> MTDSVQTETTEGKIIINLFAPNLPGSTKEDDLIQKSLRDQLVESIRNSIAYPDTDKFAGLTRFIDESGRNVFFVDGTRGAGKTTFINSVVKSLNSDQDDVKVNIKCLPTIDPTKLPRHEPILVTVTARLNKMVSDKLKGYWASNDYRKQKEQWQNHLAQLQRGLHLLTDKEYKPEYFSDALKLDAQLDYSIGGQDLSEIFEELVKRACEILDCKAILITFDDIDTQFDAGWDVLESIRKFFNSRKLVVVATGDLRLYSQLIRGKQYENYSKTLLEQEKESVRLAERGYMVEHLEQQYLLKLFPVQKRIQLKTMLQLVGEKGKAGKEEIKVKTEPGMQDIDAIDVRQAIGDAVREGLNLREGSDADMYVNELLK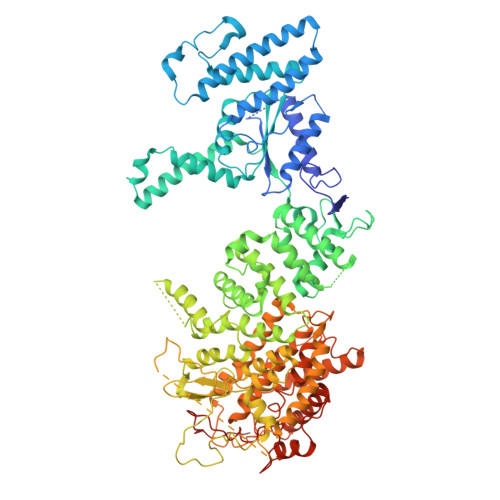QPVRLLMQVLQDFYTKKYHATSVKLDGKQSRNERPNELSVPNLLRNALYGSMLSSIYRAGLNYEQHRFGMDSLCKDIFTYVKQDRDFNTGFYLRPQSESEALRNCSIYLASQVSENCQGSLSKFLQMLLVGCGSVSIFNQFVTELARAENDREKFEQLISEYVAYMSVGRIESASHWANRCCAVVANSPNDEKIGVFLGMVQLNRKSRQHMPGGYKKFNIDTENGLAKAAMASSLSTVASNNLMDFCSVFNLIGAIADISACRCERSAITNAFNKVIAQTTCIVPPWSEAAVRAEMKGSSKSADNDAAVLDVDLDPKDDGVIDESQQDDATEFSDAITKVEQWLKNVNEIEIGIRPSALLIGKVWSRFYFNLNNVADQHKTRLYRNAEHGRMASQSNAAKIMRFNVLAFLHAVLVEESLYHSVSDREYIGEGLRLNPVTSVDEFEKKIKIIGEKLKADNKTWKNTHPLFFLLISCPILHPFIFPVGGINCSVKALNKETSFNKLIDEIVGDKLLSDEEWDYLTKNNDQKTNTRQQIFQNTITSLNSSTIVGASYDKDTPARKTKSPLLGDSEEK>[6x]HHHHHHGLIQERRSHEVNPAAHLTGANSSLTGSGGPLLWETQLGLAFLRGLSYHDGALVVTKAGYYYIYSKVQLGGVGCPLGLASTITHGLYKRTPRYPEELELLVSQQSPCGRATSSSRVWWDSSFLGGVVHLEAGEEVVVRVLDERLVRLRDGTRSYFGAFMV;>[6x]RSLPSCKEDEYPVGSECCPKCSPGYRVKEACGELTGTVCEPCPPGTYIAHLNGLSK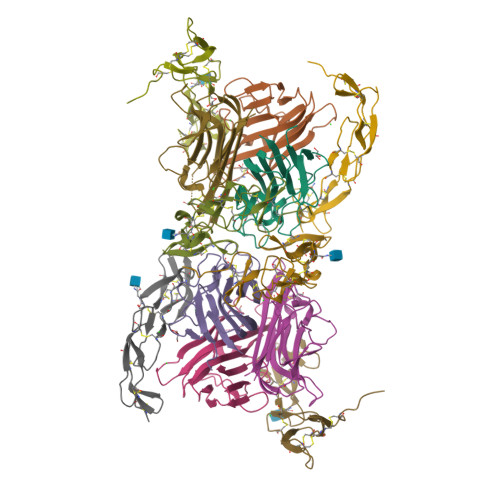CLQCQMCDPAMGLRASRNCSRTENAVCGCSPGHFCIVQDGDHCAACRAYATSSPGQRVQKGGTESQDTLCTGHHHHHH Thymidine kinase (TK) catalyses the transfer of the γ-phosphate of ATP to 2’-deoxythymidine (dThd) forming thymidine monophosphate (dTMP). L. major Type II TK (LmTK) has been previously shown to be important for infectivity of the parasite and therefore has potential as a drug target for anti-leishmanial therapy. The enzymes from Leishmania spp. are type II TKs with a ~100 amino acid C-terminal extension compared to those from other species. The overall structure of the LmTK catalytic domain in all three complexes shows a nearly identical fold to those of type II TKs from other species, as expected from the sequence identity of ~50% on the amino acid level.

Ap5dT was also a strong inhibitor of LmTK with an IC50 value of 1.1 μM. In the LmTK-AP5dT complex there are two chains in the AU, both with well-defined density for the dThd moiety and the five phosphates. The coordination of dThd is essentially identical to that in the LmTK-dTTP complex, with E85 in the inactive conformation. Only chain A exhibits good density for the adenosine, which is much less well ordered in Chain B. However, in Chain A, the adenosine is flipped by about 180° from the position expected from the CaTK and TmTK complexes, and lies on the surface of α/β-domain, partially covered by the poorly ordered 42–59 loop. In LmTK-AP5dT, the phosphates have different positions from those in the LmTK-dTTP and the TmTK-dThd-AppNHp complexes. The binding site for adenine expected from the CaTK and TmTK structures is again blocked by the adjacent dimer, just as in the LmTK-dThd complex. LmTK forms closed tetramers in all three complexes, which explains the lack of density for the adenine in LmTK-dThd and its unexpected position in LmTK-AP5dT. While hTK1 has the residues interacting with the ribose ring (D58) and the transition state (R60), these residues are disordered in most of the LmTK structures hinting at a more relaxed binding or might be a crystallographic artefact. However, it is ordered in the structure of LmTK:AP5dT with the side chain conformations of D58 and R60 being identical to hTK1. The LmTK-dThd and LmTK-AP5dT crystals contain two protomers per asymmetric unit, with the tetramer sitting on a crystallographic 2-fold axis, while the LmTK-dTTP asymmetric unit contains two tetramers.

>GPFRGRIELIIGPMFAGKTTELMRRVKREIHARRSCFVIKYSKDTRYDEHNVASHDQLMLRAQAAVSQLTEVRDTWKRFDVLAIDEGQFFSDLVDFCNTAADAGKVVMVSALDGDYRRKPFGQICELVPYCEAVDKLTAVCMMCHEQPACFTRRTVNVEQQELIGGADMYIATCRECYSKQQLP[2x]> EFL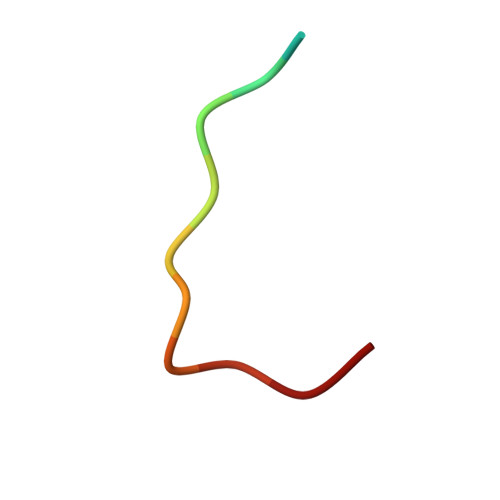PKTPIFRPD>GPAGAQDDVPPYFKTEPVRTQVHLEGNRLVLTCMAEGSWPLEFKWLHNNRELTRFSLEYRYMITSLDRTHAGFYRCIVRNRMGALLQRQTEVQVAYMGSFEEGEKRQSVNHGEAAVIRAPRISSFPRPQVTWFRDGRKIPPSSRIAITLENTLVILSTVAPDAGRYYVQAVNDKNGDNKTSQPITLAVENVGGTHEAMAPIIVVAPGNRSVVAGSSETTLECIANARPVEELSVHWKRNGVRLTSGLHSYGRRLTITNPTSADTGMYVCEATLRGSTFEPARARAFLSIIEPPYFTAEPESRILGEVEETMDIPCRAMGVPLPTLQWYKDAVPLSKLQNPRYKVLPSGGLHIQKLSPEDSGIFQCFASNEGGEVQTHTYLDVT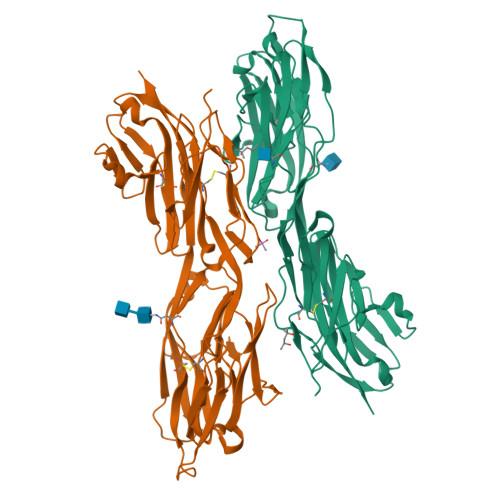N[2x]> MGKPVVAIVGRPNVGKSTIFNRIAGERISIVEDTPGVTRDRIYSSAEWLNYDFNLIDTGGIDIGDEPFLAQIRQQAEIAMDEADVIIFMVNGREGVTAADEEVAKILYRTKKPVVLAVNKLDNTEMRANIYDFYSLGFGEPYPISGTHGLGLGDL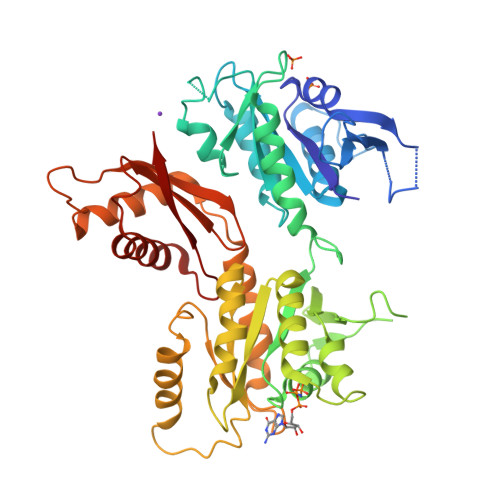LDAVAEHFKNIPETKYNEEVIQFCLIGRPNVGKSSLVNAMLGEERVIVSNVAGTTRDAVDTSFTYNQQEFVIVDTAGMRKKGKVYETTEKYSVLRALKAIDRSEVVAVVLDGEEGIIEQDKRIAGYAHEAGKAVVIVVNKWDAVDKDESTMKEFEENIRDHFQFLDYAPILFMSALTKKRIHTLMPAIIKASENHSLRVQTNVLNDVIMDAVAMNPTPTHNGSRLKIYYATQVSVKPPSFVVFVNDPELMHFSYERFLENRIRDAFGFEGTPIKIFARARK>MEHKRGHVLAVPYPTQGHITPFRQFCKRLHFKGLKTTLALTTFVFNSINPDLSGPISIATISDGYDHGGFETADSIDDYLKDFKTSGSKTIADIIQKHQTSDNPITCIVYDAFLPWALDVAREFGLVATPFFTQPCAVNYVYYLSYINNGSLQLPIEELPFLELQDLPSFFSVSGSYPAYFEMVLQQFINFEKADFVLVNSFQELELHENELWSKACPVLTIGPTIPSIYLDQRIKSDTGYDLNLFESKDDSFCINWLDTRPQGSVVYVAFGSMAQLTNVQMEELASAVSNFSFLWVVRSSEEEKLPSGFLETVNKEKSLVLKWSPQLQVLSNKAIGCFLTHCGWNSTMEALTFGVPMVAMPQWTDQPMNAKYIQDVWKAGVRVKTEKESGIAKREEIEFSIKEVMEGERSKEMKKNVKKWRDLAVKSLNEGGSTDTNIDTFVSRVQSK[2x]

UGT74F1 and UGT74F2 are the enzymes responsible for the in vivo glucosylation of SA in A. thaliana. In UGT74F1, glucose is transferred to the hydroxyl of SA, creating a glucoside; in UGT74F2, glucose is transferred to the carboxylate group of SA to create a glucose ester. UGT74F2 exhibits the GT-B fold with ligands bound in the cleft between the two domains –the N-terminal domain is comprised of residues 1–245, while 246–449 make up the C-terminal domain. UDP and SA interact primarily with residues in the C- and N-terminal domain, respectively.

To verify the presence of a single SA in the binding domain, we co-crystallized UGT74F2 with the SA analog 2-BA. Collection of an anomalous X-ray diffraction set showed a single anomalous peak in the SA binding pocket. While there is partial overlap between 2-BA and SA binding sites, the location of the carboxyl group of 2-BA differs from that of SA and is within hydrogen bond interaction from Thr 365. Over 300 crystals were screened and, generally, co-crystallization of the protein with UDP/UDP-glucose and SA produced a smaller fraction of well-diffracting crystals (diffraction resolution up to 2.5 Å, ~5%) than the protein co-crystallized with UDP/UDP-glucose and 2-BA (~60%). Therefore, we propose that SA binds to UGT74F2 primarily in the conformation described for the UDP/SA complex (i.e. carboxyl group of SA interacting with His 18 and Thr 15) but binds to UGT74F1 primarily in the conformation modeled on the basis of 2-BA in the 2-BA/UDP complexes of UGT74F2 wild-type or T15S (i.e. SA hydroxyl interacting with His 18 and SA carboxyl interacting with Thr 365).> MYVASWQDYHSDFSEKYGDIALKKKLEQNTKKLDEESSQLETTTRSIDSADDLDQFIKNYLDIRTQYHLRREK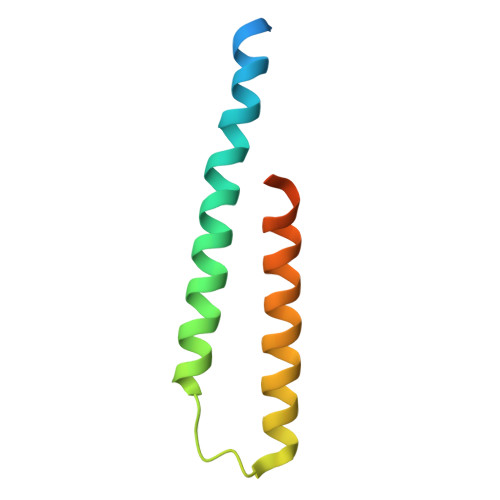LATWDKQGNLKY> MAHHHHHHSLSSPYILVLYYSRHGATAEMARQIARGVEQGGFEARVRTVPAVSTECEAVAPDIPAEGALYATLEDLKNCAGLALGSPTRFGNMASPLKYFLDGTSSLWLTGSLVGKPAAVFTSTASLHGGQETTQLSMLLPLLHHGMLVLGIPY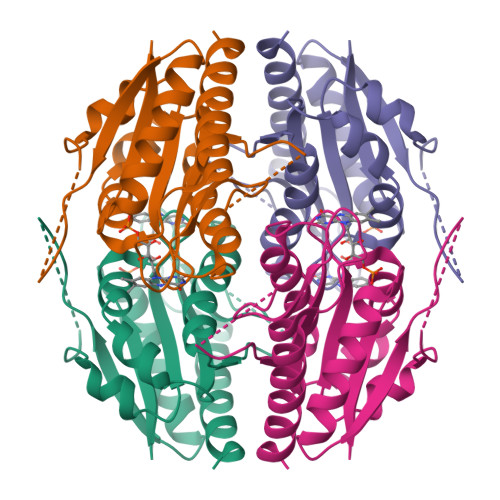SEPALLETRGGGTPYGASHFAGADGKRSLDEHELTLCRALGKRLAETAGKLEG2-[4-[3,5-bis(trifluoromethyl)phenyl]phenyl]ethanoic acid | C16 H10 F6 O2 | 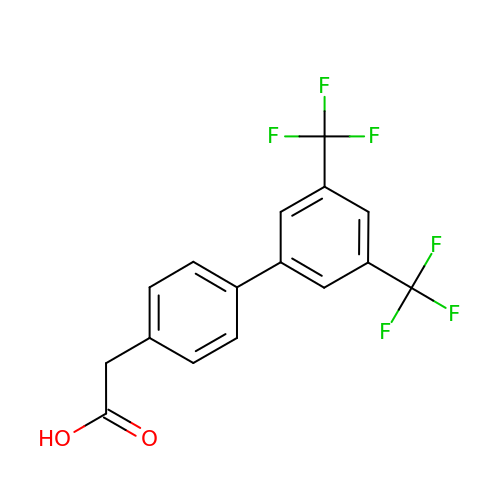QXUJSELRLOECDC-UHFFFAOYSA-N>MATLQDIGVSAGINILSAFVFFIIFAVLRLQPFNDRVYFSKWYLKGLRSSPARGGAFAQRFVNLDFRSYMKFLNWMPEALKMPEPELIDHAGLDSVVYLRIYWLGLKIFTPIAVLAWAVLVPVNWTNNTLEMAKQLRNVTSSDIDKLSVSNIPEYSMRFWTHIVMAYAFTIWTCYVLMKEYETIANMRLQFVASEARRPDQFTVLVRNVPPDADESVSELVEHFFLVNHPDHYLTHQVVCNANKLADLVKKKKKLQNWLDYYQLKYARNNSQRIMVKLGFLGLWGQKVDAIEHYIAEIDKISKEISKEREEVVNDPKAIMPAAFVSFKTRWAAAVCAQTQQTRNPTQWLTEWAPEPRDVFWSNLAIPYVSLTVRRLIMHVAFFFLTFFFIVPIAFVQSLATIEGIVKAAPFLKFIVDDKFMKSVIQGFLPGIALKLFLAFLPSILMIMSKFEGFTSISSLERRAAFRYYIFNLVNVFLASVIAGAAFEQLNSFLNQSANQIPKTIGVAIPMKATFFITYIMVDGWAGVAGEILMLKPLIMFHLK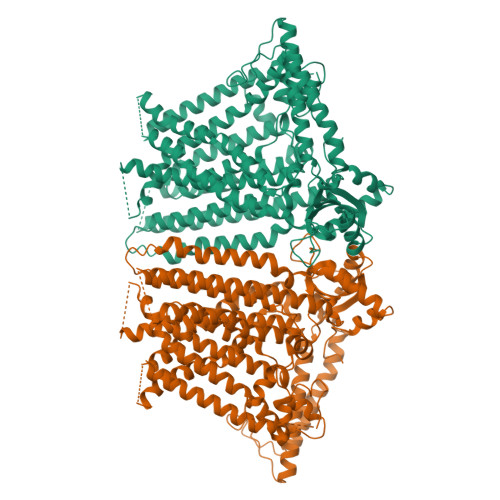NAFLVKTDKDREEAMDPGSIGFNTGEPRIQLYFLLGLVYAPVTPMLLPFILVFFALAYIVYRHQIINVYNQEYESAAAFWPDVHGRVIAALVISQLLLMGLLGTKHAALAAPFLIALPVLTIGFHHFCKGRYEPAFIRYPLQEAMMKDTLETAREPNLNLKGYLQNAYVHPVFKGDEDDYDIDDKLGKFEDEAIIVPTKRQSRRNTPAPSIISGDDSPSLPFSGKLVGTGTLEVLFQ[2x]>AESTLGAAAAQSGRYFGTAIASGKLGDSAYTTIASREFNMVTAENEMKIDATEPQRGQFNFSAGDRV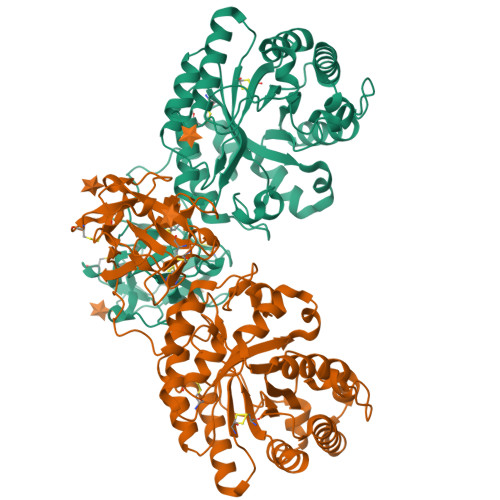YNWAVQNGKQVRGHTLAWHSQQPGWMQSLSGSTLRQAMIDHINGVMGHYKGKIAQWDVVNEAFSDDGSGGRRDSNLQRTGNDWIEVAFRTARAADPAAKLCYNDYNIENWTWAKTQGVYNMVRDFKQRGVPIDCVGFQSHFNSGSPYNSNFRTTLQNFAALGVDVAITELDIQGASSSTYAAVTNDCLAVSRCLGITVWGVRDTDSWRSGDTPLLFNGDGSKKAAYTAVLNALNGGSSTPPPSGGGQIKGVGSGRCLDVPNASTTDGTQVQLYDCHSATNQQWTYTDAGELRVYGDKCLDAAGTGNGTKVQIYSCWGGDNQKWRLNSDGSIVGVQSGLCLDAVGGGTANGTLIQLYSCSNGSNQRWTRT[2x]> DYKDDDDKAEVKKIPTMIEGFDDISHGGLPQGATTLVSGTSGTGKTLFAVQFLYNGITIFNEPGIFVTFEESPQDIIKNALSFGWNLQSLIDQGKLFILDASPDPDGQEVAGDFDLSALIERIQYAIRKYKATRVSIDSVTAVFQQYDAASVVRREIFRLAFRLAQLGVTTIMTTERVDEYGPVARFGVEEFVSDNVVILRNVLEGERRRRTVE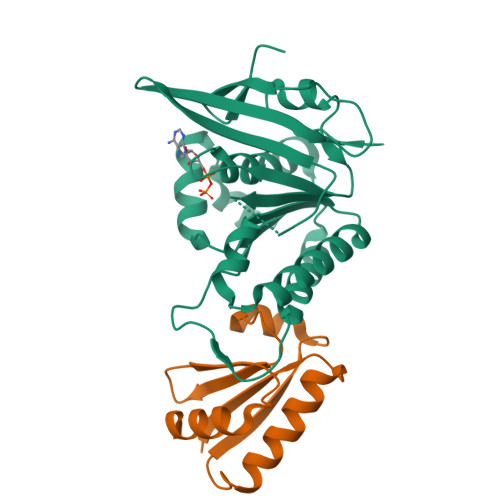ILKLRGTTHMKGEYPFTINNGINIFDYKDDDDK;> MAPLRKTAVLKLYVAGNTPNSVRALKTLNNILEKEFKGVYALKVIDVLKNPQLAEEDKILATPTLAKVLPPPVRRIIGDLSNREKVLIALRLLAEEIGD> GAMGESLSIYKSGLKNDFQDWSWGEHSLTDTTNVESGETNSISFTPKAYGAVFLGCFECIDTDTYNNIEFDINGGSSGAQLLRITVVKNSKSVGSKLITDLNGGTPIEANSWTKIKASFIDDFKVSGKVDGIWIQDIKGDTQSTVYISNIIATA

Here, we present the first crystallographic structure of a CBM8 family member (CBM8), DdCBM8, from the slime mold Dictyostelium discoideum, which was identified attached to an endo-β-1,4-glucanase (glycoside hydrolase family 9). DdCBM8 is located at the C-terminal region of CelA and is connected to the catalytic GH9 domain through a threonine–glutamate–threonine–proline repeat linker. We show that the planar carbohydrate-binding site of DdCBM8, composed of aromatic residues, is similar to type A CBMs that are specific for crystalline (multichain) polysaccharides. However, affinity gel electrophoresis demonstrated that DdCBM8 also bound to soluble (single chain) polysaccharides, especially glucomannan, similar to type B CBMs, although it had no apparent affinity for oligosaccharides.

Initial phases were determined using the single-wavelength anomalous dispersion method using anomalous scattering of iodine, as described in the Experimental procedures section. At the end of refinement, the derivative dataset (resolution of 1.8 Å) displayed 13 iodine atoms with occupancies varying from 0.42 to 0.83.> GNIQVKNASELNKAIGSAVAGDAILMQPGEWKDVKILFNSKASKAKPITLKADQAGKVMLSGESSLSFDAPYLVVEGLLFKDGSLKKGSVIQFNSDYCKLENTAIVDFNPSQKSTGYYWVLFRGNNNLMQYCSFKGKNNMQPLVGNDQDNSRYNTVQYCYFKDIPYTPDNGREIFRIWGYGRSEETGDDGAFFTIKNNLFERAHGEGMEIISLKSNRNKVIGNTVISTKGGIVGRSGNFNTIEENFIFGENEKGSYGIRLAGQGHHVVNNYVRDVDGDGLILICGEYIEKALTDKYEPILRAGTPLGRVPRYGHVKDGLYVNNTFLNVGGAGINIGGSYNGNPGADQRMLLPENNTITHNIISTKSGKNAIQATSPSQNPILANFKFKSNILGSNLVYDNGAE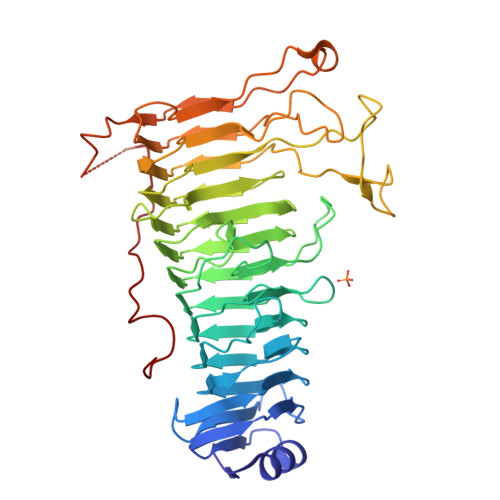PDSGVKETPITINGKEYKIPFASKKDTLITSKPGVRIKNKPLSSKEVGVKWSI>[4x]AEEFPVPNGFESAYREVDGVKLHYVKGGQGPLVMLVHGFGQTWYEWHQLMPELAKRFTVIAPDLPGLGQSEPPKTGYSGEQVAVYLHKLARQFSPDRPFDLVAHDIGIWNTYPMVVKNQADIARLVYMQAPIPDARIYRFPAFTAQGESLVWHFSFFA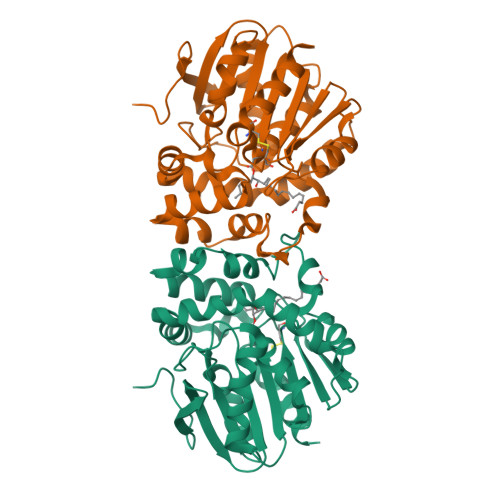ADDRLAETLIAGKERFFLEHFIKSHASNTEVFSERLLDLYARSYAKPHSLNASFEYYRALNESVRQNAELAKTRLQMPTMTLAGGGHGGMGTFQLEQMKAYAEDVEGHVLPGCGHWLPEECAAPMNRLVIDFLSRGRHHHHHH> SMKAEEARLEGKEYFTKSDWPNAVKAYTEMIKRAPEDARGYSNRAAALAKLMSFPEAIADCNKAIEKDPNFVRAYIRKATAQIAVKEYASALETLDAARTKDAEVNNGSSAREIDQLYYKAS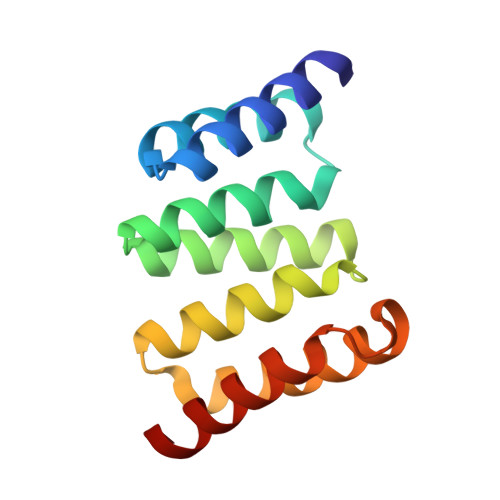QQRF N-[(1R)-2,3-dihydro-1H-inden-1-yl]adenosine 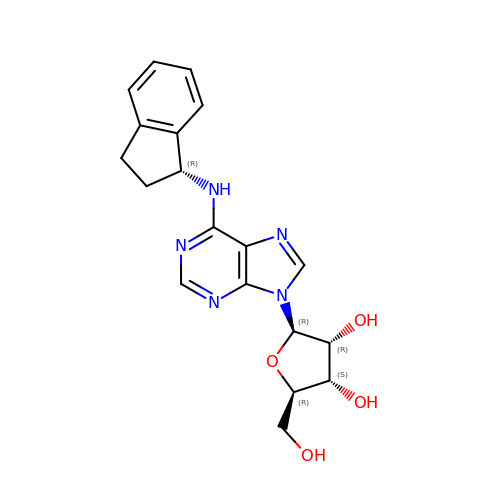| C19 H21 N5 O4 | FSKMJUWPFLDDRS-BYMDKACISA-N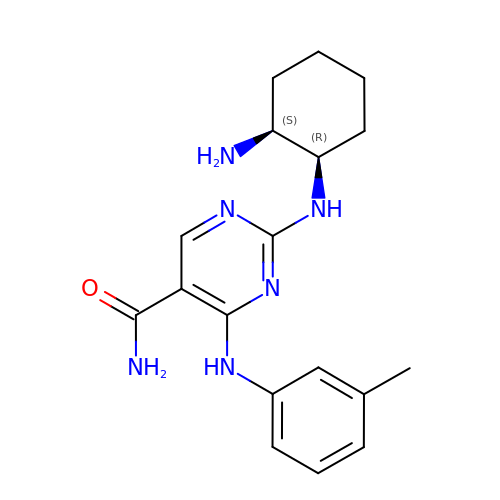2-{[(1R,2S)-2-aminocyclohexyl]amino}-4-[(3-methylphenyl)amino]pyrimidine-5-carboxamide | C18 H24 N6 O | NZNTWOVDIXCHHS-LSDHHAIUSA-N> ALVKEEIQAKEYLENLNKELAKRTNVETEAAWAYGSNITDENEKKKNEISAELAKFMKEVASDTTKFQWRSYQSEDLKRQFKALTKLGYAALPEDDYAELLDTLSAMESNFAKVKVCDYKDSTKCDLALDPEIEEVISKSRDHEELAYYWREFYDKAGTAVRSQFERYVELNTKAAKLNNFTSGAEAWLDEYEDDTFEQQLEDIFADIRPLYQQIHGYVRFRLRKHYGDAVVSETGPIPMHLLGNMWAQQWSEIADIVSPFPEKPLVDVSAEMEKQGYTPLKMFQMGDDFFTSMNLTKLPQDFWDKSIIEKPTDGRDLVCHASAWDFYLTDDVRIKQCTRVTQDQLFTVHHELGHIQYFLQYQHQPFVYRTGANPGFHEAVGDVLSLSVSTPKHLEKIGLLKDYVRDDEARINQLFLTALDKIVFLPFAFTMDKYRWSLFRGEVDKANWNCAFWKLRDEYSGIEPPVVRSEKDFDAPAKYHISADVEYLRYLVSFIIQFQFYKSACIKAGQYDPDNVELPLDNCDIYGSAAAGAAFHNMLSMGAS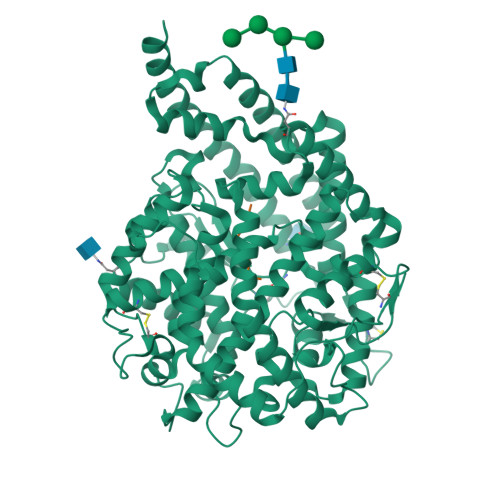KPWPDALEAFNGERIMSGKAIAEYFEPLRVWLEAENIKNNVHIGWTTSNKCVS;> EGLPPRPKIPP> GPLGSAHKLFIGGLPNYLNDDQVKELLTSFGPLKAFNLVKDSATGLSKGYAFCEYVDINVTDQA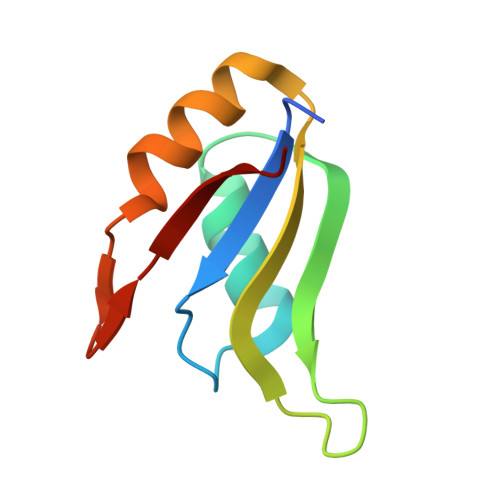IAGLNGMQLGDKKLLVQRAS> MALDVKKYPFIKSLDDELKKYGGGITLTDLLLNSTTLIDQAKDRIQKTKSGDELPHYVSYNEPVLVFYTTLLSLAILNDVKLIRRYAYAEAKQFRSLLHTENEENLLEISKLLDLKINRCDPIKFYLEKKRRIIQKEFCVHFIDYLKYTKDLKEDWKLSGQILHKGYVYLDKNQLIGLIAESIKSKIVEMIRPLNLKEIPEKLKSLIERRGIIPPCIENILAKEKLNEEEIRTLITFYIDIGKGLSGIVSIMKKYNVSNVEDLYRKYRGDKGTRYIVYSCAKMKQLGL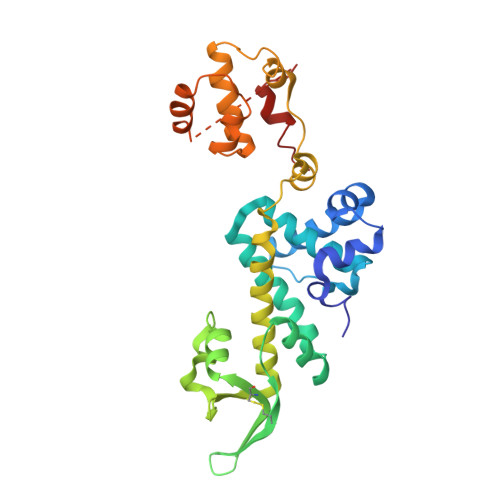CVSSCNVKNPLQLYFLSNE>MATEGGGKEMNEIKTQFTTREGLYKLLPHSEYSRPNRVPFNSQGSNPVRVSFVNLNDQSGNGDRLCFNVGRELYFYIYKGVRKAADLSKPIDKRIYKGTQPTCHDFNHLTATAESVSLLVGFSAGQVQLIDPIKKETSKLFNEERLIDKSRVTCVKWVPGSESLFLVAHSSGNMYLYNVEHTCGTTAPHYQLLKQGESFAVHTCKSKSTRNPLLKWTVGEGALNEFAFSPDGKFLACVSQDGFLRVFNFDSVELHGTMKSYFGGLLCVCWSPDGKYIVTGGEDDLVTVWSFVDCRVIARGHGHKSWVSVVAFDPYTTSVEEGDPMEFSGSDEDFQDLLHFGRDRANSTQSRLSKRNSTDSRPVSVTYRFGSVGQDTQLCLWDLTEDILFPHQPLSRARTHTNVMNATSPPAGSNGNSVTTPGNSVPPPLPRSNSLPHSAVSNAGSKSSVMD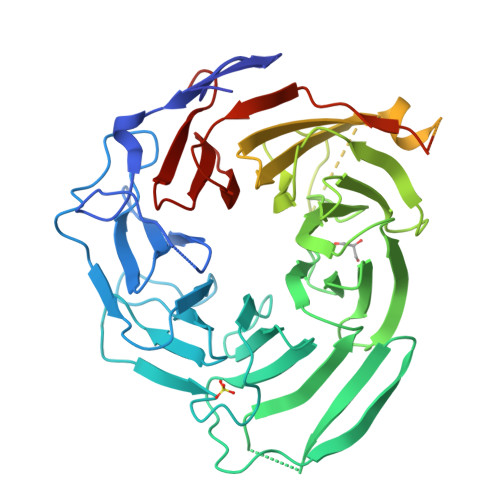GAIASGVSKFATLSLHDRKERHHEKDHKRNHSMGHISSKSSDKLNLVTKTKTDPAKTLGTPLCPRMEDVPLLEPLICKKIAHERLTVLIFLEDCIVTACQEGFICTWGRPGKVVSFNP[3x]>[4x]MDKPLKLYFIPYLAAGHMIPLCDIAALFASRGHFVTIITTPLNAKILPKYNNFNVHTFQFPSQEVGLPEGVENLSAVTDLDGAYKIYQAMALLREHIENFVEQHPPDCIVADFLLPWVDELANKLSIPRLAFNGFSLFTICAME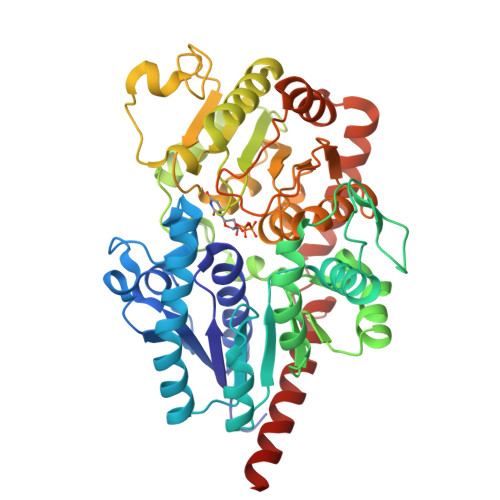SLRSHPLPEDASGPFVIPNFPQDIVINSTPPAESKTFMDPLFTIALKSNGFIINSFVEFDGEEYVKYYEKTIGHKAWHLGPASLVRETIQEKAERGEKSTLSVQKFVDWLNKKRDNSVIYISFGTMCHFPDKQLFEIASAIEASGYDFIWVVPEKKGKENESEDDKEKWLPKGFEERDNGMIVKGWSPQMVILGHPAVGAFLTHCGWNSTVEAVSAGVPMITWPVLGDQFYNEKLITQVRGIGVEVGVDEWVVTSFRGMKQLVGRDCIEKAIRRLMDGGDEAIQIRERSQKLAKITKHVVQEGGSSYENLTVLINELKQLRDCKVLN> GAHMGNWATHVYVPYEAKEEFLDLLDVLLPHAQTYVPRLVRMKVFHLSLSQSVVLRHHWILPFVQALKARMTSFHRFFFTANQVKIYTNQEKTRTFIGLEVTSGHAQFLDLVSEVDRVMEEFNLTTFYQDPSFHLSLAWCVGDARLQLEGQCLQELQAIVDGFEDAEVLLRVHTEQVRCKSGNKFFSMPLK

Usb1 is an exoribonuclease that shortens the oligo-uridine tail of U6 snRNA, resulting in a terminal 2′,3′ cyclic phosphate group in most eukaryotes, including humans. Usb1 is a member of the 2H phosphodiesterase superfamily, a large enzyme family containing members with known 2′,3′-cyclic or 1″,2″-cyclic phosphodiesterase (CPDase) activity, or 3′-5′ or 2′-5′ phosphodiesterase activity, or 2′,5′-RNA ligase activity. The active sites of 2H phosphodiesterase enzymes are characterized by a symmetric shape with two HxT/S motifs centered in a catalytic cleft. We report three high-resolution co-crystal structures of Usb1 complexed with RNA, which show the structural basis for this catalytic preference and unambiguously identify His120 and His208 as catalytic base and acid, respectively.

In order to visualize how adenosine binds in the unperturbed active site, we crystallized wild-type Usb1 with the substrate mimic adenosine 5′-monophosphate (AMP). AMP bound in the n pocket, with His208 well-positioned to act as a catalytic acid to protonate the leaving group 5′ oxygen of the terminal nucleotide. His208 is also hydrogen bonded to the backbone oxygen of Ser206. In the wt–AMP structure, Ser210 (part of the HxS catalytic motif) helps orient the scissile phosphate by forming a 2.7 Å hydrogen bond to one of the non-bridging oxygens. The syn conformation also allows a water molecule to hydrogen bond to both the AMP N3 nitrogen and the non-bridging oxygen of the scissile phosphate. Coordination of this water molecule may help stabilize an in-line conformation of the scissile phosphate. Comparison of the AMP-bound structure with our previously determined UMP-bound structure shows that UMP cannot coordinate a water molecule in a similar fashion. We also observe that, relative to the UMP bound structure, AMP makes a shorter hydrogen bond between the hydroxyl group of Ser210 and the scissile phosphate. These unique features of AMP bound to the n pocket may provide a rationale as to why the enzyme is more efficient at cleaving a terminal adenosine relative to uridine.> SMDDDDQVAFSFILDNIVTQKMMAVPDSWPFHHPVNKKFVPDYYKVIVNPMDLETIRKNISKHKYQSRESFLDDVNLILANSVKYNGPESQYTKTAQEIVNVCYQTLTEYD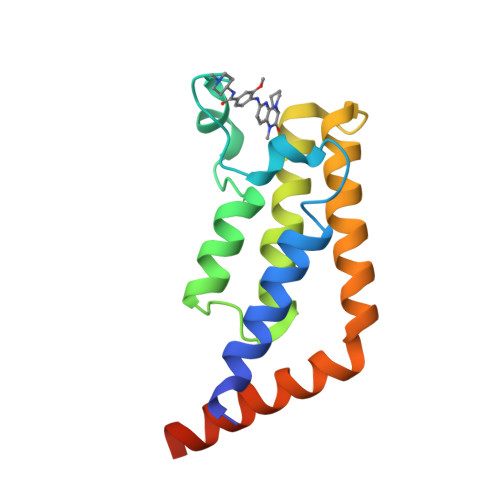EHLTQLEKDICTAKEAALEEAELESLD> CCUGAGUUCAAU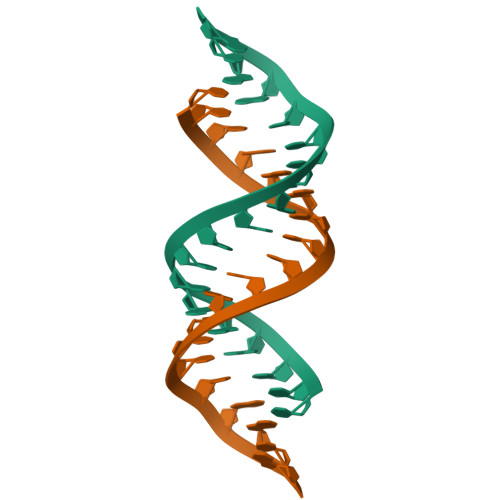UCUAGCG>GSHMDYNKRSSVSTVPNAAPIRVGFVGLNAAKGWAIKTHYPAILQLSSQFQITALYSPKIETSIATIQRLKLSNATAFPTLESFASSSTIDMIVIAIQVASHYEVVMPLLEFSKNNPNLKYLFVEWALACSLDQAESIYKAAAERGVQTIISLQGRKSPYILRAKELISQGYIGDINSIEIAGNGGWYGYERPVKSPKYIYEIGNGVDLVTTTFGHTIDILQYMTSSYFSRINAMVFNNIPEQELIDERGNRLGQRVPKTV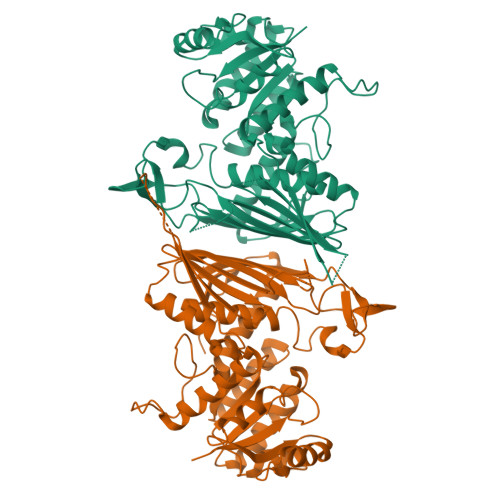PDHLLFQGTLLNGNVPVSCSFKGGKPTKKFTKNLVIDIHGTKRDLKLEGDAGFAEISNLVLYYSGTRANDFPLANGQQAPLDPGYDAGKEIMEVYHLRNYNAIVGNIHRLYQSISDFHFNTKKIPELPSQFVMQGFDFEGFPTLMDALILHRLIESVYKSNMMGSTLNVSNISHYSL[2x]> GSAAASPAWMPAYACQRPTPLTHHNTGLSEALEILAEAAGFEGSEGRLLTFCRAASVLKALPSPVTTLSQLQGLPHFGEHSSRVVQELLEHGVCEEVERVRRS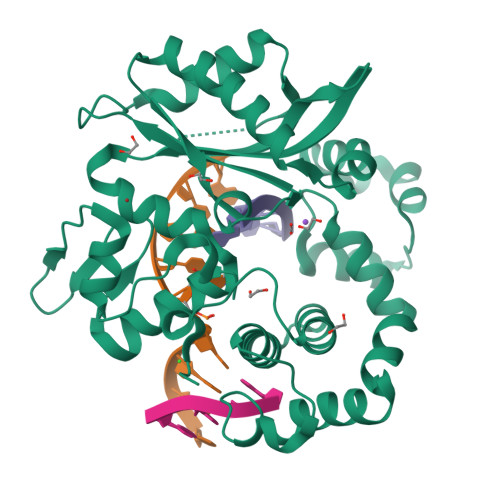ERYQTMKLFTQIFGVGVKTADRWYREGLRTLDDLREQPQKLTQQQKAGLQHHQDLSTPVLRSDVDALQQVVEEAVGQALPGATVTLTGGFRRGKLQGHDVDFLITHPKEGQEAGLLPRVMCRLQDQGLILYHQHQHSCCESPTRLAQQSHMDAFERSFCIFRLPQPGSWKAVRVDLVVAPVSQFPFALLGWTGSKLFQRELRRFSRKEKGLWLNSHGLFDPEQKTFFQAASEEDIFRHLGLEYLPPEQRNA> MIHFILLFSRQGKLRLQKWYITLPDKERKKITREIVQIILSRGHRTSSFVDWKELKLVYKRYASLYFCCAIENQDNELLTLEIVHRYVELLDKYFGNVCELDIIFNFEKAYF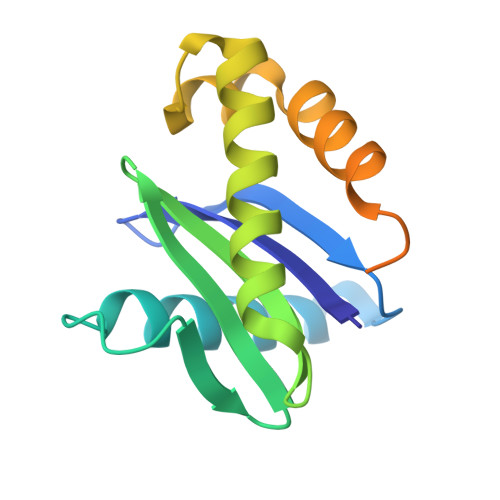ILDEFIIGGEIQETSKKIAVKAIEDSDMLQEVSTVSQTMGER The reductive dehalogenases (RDases) are key enzymes in organohalide respiration, which is performed by a unique subset of bacteria. The RDases are cobalamin-dependent and able to selectively cleave carbon-halogen bonds through reduction. The RDases can be split into two classes: (i) the canonical respiratory dehalogenases, which use a halogenated compound as a final electron acceptor during organohalide respiration and (ii) the catabolic respiratory dehalogenases that occur in the catabolic pathways of non-organohalide respiring bacteria. Structural insight into RDase function is based on two enzymes that have been crystallised, the respiratory perchloroethene (PCE) Sulfurospirillum multivorans reductive dehalogenase (PceA), and the catabolic reductive dehalogenase from Nitratireductor pacificus pht-3B (NpRdhA).

The NpRdhA variant K488Q was previously reported to lack 35-DB-4-OH reductase activity. Crystals of the K488Q variant were obtained in the same condition as the wild type NpRdhAN crystals. Alignment of chain A of K488Q and the NpRdhAN structure gave an rmsd of 0.179 over 680 residues. The only major difference occurred, as expected, at position Q488. An overlay of the three K488Q NpRdhA monomers reveals multiple conformations of Q488 and adjacent residues S422 and R552, also implicated in substrate binding. The K488Q crystal structure confirms that no significant changes occur to the wider protein active site. EPR analysis of the K488Q variant reveals a sharpening of spectral features upon addition of substrate, but not the clear cobalt-halogen interaction seen with WT NpRdhA, suggesting non-productive binding with water remaining as the fifth ligand to the cobalt ion. Thus, it seems that the K488Q mutation disrupts the halide ion and substrate binding properties of the active site, likely a consequence of the disorder induced at positions S422 and R552, as well as perturbation of the Tyr426 pKa. The extent by which the K488Q mutation disrupts substrate binding casts light on the critical role K488 plays in this enzyme. Unfortunately, crystal structures of K488Q ligand complexes could not be obtained, despite several attempts.

>[3x]MVQTSFEHHHHHHSAGENLYFQGAQISMRLYSNRDRPNHLGPLALERLARVDDVVAQPARQPEDGFAASEDSLLGDVEEYARLFTRFLDGPVAPLGDAIPDDPARRAENLKASAYFLDASMVGICRLDPDDRAGDCDPSHTHALVFAVQFGREPEAGEAGAEWIRGTNAARTDMRCAEIAAILSGYVRWMGFPARGHFSGDAQVDLARLAVRAGLARVVDGVLVAPFLRRGFRLGVVTTGYALAADRPLAPEGDLGETAPEVMLGIDGTRPGWEDAEEEKRPLHMGRYPMETIRRVDEPTTLVVRQEIQRVAKRGDFFKRAEAGDLGEKAKQEKKRFPMKHPLALGMQPLIQNMVPLQGTREKLAPTGKGGDLSDPGRNAEAIKALGYYLGADFVGICRAEPWMYYASDEVEGKPIEAYHDYAVVMLIDQGYETMEGASGDDWISASQSMRAYMRGAEIAGVMAAHCRRMGYSARSHSNAHSEVIHNPAILMAGLGEVSRIGDTLLNPFIGPRSQSIVFTTDLPMSVDRPIDFGLQDFCNQCRKCARECPCNAISFGDKVMFNGYEIWKADVEKCTKYRVTQMKGSACGRCMKMCPWNREDTVEGRRLAELSIKVPEARAAIIAMDDALQNGKRNLIKRWWFDLEVIDGVAGAPRMGTNERDLSPDRGDKIGANQKLAMYPPRLQPPPGTTLDAVLPVDRSGGLAEYAAAETPAAARARLKSSAG>MASMQPPIAKPGETWILQAKRSDEFNVKDATKWNFQTENYGVWSWKNENATVSNGKLKLTTKR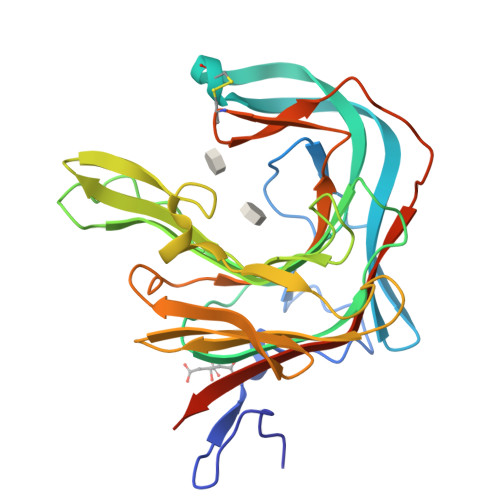ESHQRTFWDGCNQQQVANYPLYYTSGVAKSRATGNYGYYEARIKGASTFPGVSPAFWMYSTIDRSLTKEGDVQYSEIDVVDLTQKSAVRESDHDLHNIVVKNGKPTWMRPGSFPQTNHNGYHLPFDPRNDFHTYGVNVTKDKITWYVDGEIVGEKDNLYWHRQMNLTLSQGLRAPHTQWKCNQFYPSANKSAEGFPTSMEVDYVRTWVKVGNNNLEHHHHHH[2x]>[6x]MSELFSERIPPQSIEAEQAVLGAVFLDPAALVPASEILIPEDFYRAAHQKIFHAMLRVADRGEPVDLVTVTAELAASEQLEEIGGVSYLSELADAVPTAANVEYYARIVEEKSVLRRLIRTATSIAQDGYTREDEIDVLLDEADRKIMEVSQRKHSGAFKNIKDILVQTYDNIEMLHNRDGEITGIPTGFTELDRMTSGFQRSDLIIVAARPSVGKTAFALNIAQNVATKTNENVAIFSLEMSAQQLVMRMLCAEGNINAQNLRTGKLTPEDWGKLTMAMGSLSNAGIYIDDTPSIRVSDIRAKCRRLKQESGLGMIVIDYLQLIQGSGRSKENRQQEVSEISRSLKALARELEVPVIALSQLSRSVEQRQDKRPMMSDIRESGSIEQDADIVAFLYRDDYYNKDSENKNIIEIIIAKQRNGPVGTVQLAFIKEYNKFVNLERRFDEAQIPPGA;>KLLPAFQNAERLLLAHMMRSRDVALVVQERIGGRFNIEEHRALAAYIYAFYEEGHEADPGALISRIPGELQPLASELSLLLIADDVSEQELEDYIRHVLNRPKWLMLKVKEQEKTEAERRKDFLTAARIAKEMIEMKKMLSSS[3x];>[6x]MEPIGRSLQGVTGRPDFQKRLEQMKEKVMKDQDVQAFLKENEEVIDQKMIEKSLNKLYEYIEQSKNCSYCSEDENCNNLLEGYHPKLVVNGRSIDIEYYECPVKRKLDQQKKQQSLMKSMYIQQDLLGATFQQVDISDPSRLAMFQHVTDFLKSYNETGKGKGLYLYGKFGVGKTFMLAAIANELAEKEYSSMIVYVPEFVRELKNSLQDQTLEEKLNMVKTTPVLMLDDIGAESMTSWVRDEVIGTVLQHRMSQQLPTFFSSNFSPDELKHHFTYSQRGEKEEVKAARLMERILYLAAPIRLDGENRRHPHHHHHH

The replicative hexameric DnaB helicase is composed of two domains that are connected by one flexible linker. The larger CTD exhibits a classical RecA fold, binds the nucleoside triphosphate and translocates the protein on the DNA, whereas the NTD surrounds the single-stranded DNA (ssDNA) during DNA unwinding and binds the primase1920. The DnaI helicase loader belongs to the AAA+ family of ATPases2526. Here we report a crystal structure of BstDnaB helicase in complex with BsuDnaI loader protein and the HBD of BstDnaG primase at 7.5 Å resolution.

The overall architecture of the 570-kDa complex exhibits a three-layered ring structure along the c axis of the crystal. The NTDs of BstDnaB together with the HBDs of BstDnaG form the first ring that lies on the top of the second ring, which consists of the CTDs of BstDnaB. The NTDs of BstDnaB pack into a more rigid triangular collar shape that exhibits a threefold symmetry, whereas the CTDs have a relatively loose collar shape with a pseudo sixfold symmetry. The BsuDnaI on the bottom forms the loosest triangular collar of trimer of dimers with an obvious threefold symmetry as well. The diameter of the central channel is around 50–55 Å throughout its length, which is wide enough to allow either double-stranded DNA or ssDNA to pass through the channel. The CTDs of hexameric BstDnaB helicase interact with both the NTDs and the CTDs of the helicase loader BsuDnaI with a total contact surface area of ~1,745 Å2 per hexamer. Therefore, it appears that the NTDs of BsuDnaI have the major role in recruiting the helicase loader into the prepriming complex. The CTDs of one dimer (chains N and O) exhibit a different orientation from the others and do not directly interact with the CTDs of the helicase. Moreover, the structure and the proposed model suggest that the release of helicase loaders may result from the binding of ssDNA to the helicase ring, which is accompanied by the shift from the ‘open-ring’ to the ‘open-spiral’, and then the ‘closed-spiral’ state of the helicase ring.1-beta-D-glucopyranosyl-4-phenyl-1H-1,2,3-triazole | C14 H17 N3 O5 | 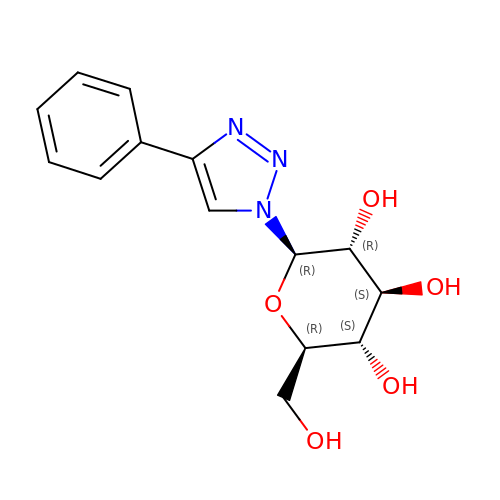SLCZDPXCZLKLKY-RKQHYHRCSA-N> HHHMRIEVKLLPLKDNPILPFNYNYEVYSQILEKVNSIEPTIAKLLSSPHGFWTFSRIIVRKRKILPDKGIEILSDDVSLYISSSNEDIIRAIAEAVEKSPEFKIGELSFLVGDIKAI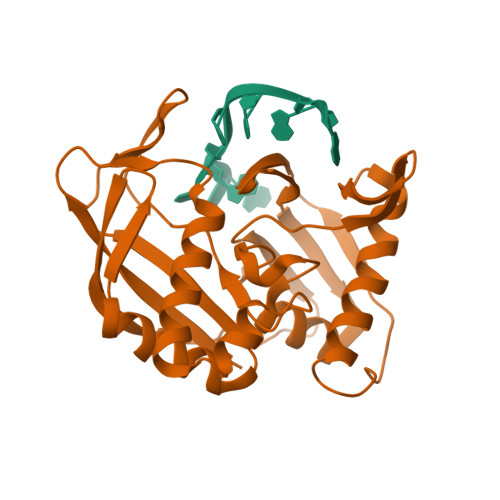KVKELGKENVFSTLSPIVVRTVKFEGNKLRHWDLYPHDELFMDRLRKVMILRYSEVMGETPKDRDFTIEVLKFKPTRLMVGSSYIRGSLMVFRYAGSEEIARFGYENGFGEKTGLGFGMVKLIE>[2x]DPTLEWFLSHCHIHKYPSKSTLIHQGEKAETLYYIVKGSVAVLIKDEEGKEMILSYLNQGDFIGELGLFEEG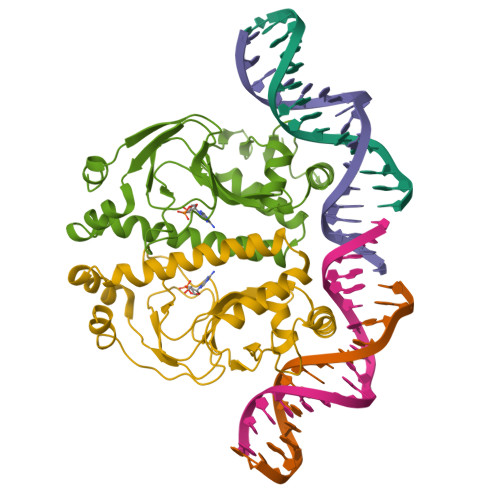QERSAWVRAKTACEVAEISYKKFRQLIQVNPDILMRLSAQMARRLQVTSEKVGNLAFLDVTGRIAQTLLNLAKQPDAMTHPDGMQIKITRQEIGQIVGCSRETVGRILKMLEDQNLISAHGKTIVVYG> MASMTGGQQMGRDEAGITGTWYNQLGSTFIVTAGADGALTGTYESAVGNAESRYVLTGRYDSAPATDGSGTALGWTVAWKNNYRNAHSATTWSGQYVGGAQARINTQWLLTYGTTEANAWASTLVGHDTFTKVKPSAASIDAAKKAGVNNGNPLDAVQQ

Our work utilizes biotin–streptavidin (Sav) technology to develop artificial metalloproteins (ArMs) that mimic the active sites of natural copper metalloenzymes. Our group develops artificial metalloproteins (ArMs) using biotin–streptavidin (Sav) technology to mimic natural metalloenzyme active sites to characterize otherwise elusive intermediates and study the effects of the secondary coordination sphere on metal ion(s) reactivity. This approach leverages the strong binding affinity between biotinylated metal complexes and the Sav host to confine synthetic metal cofactors within a protein scaffold. By engineering ArMs with aromatic residues within their secondary coordination spheres, we systematically investigate the influence of these residues on Cu reactivity and oxidant activation. Our results demonstrate how the inclusion of aromatic residues within the secondary coordination sphere influences the structure and reactivity of copper ArMs.

We reasoned that a tyrosine mutation at position S112 would be close enough to our Cu cofactors to influence the structure and reactivity but would not be oriented to participate in direct coordination. To prepare this type of Cu ArM, a triple mutant variant of Sav, referred to as 2XM-S112Y-Sav, was engineered; this mutant contains S112Y and two additional mutations, K121A and E101Q, which we have found to prevent unwanted interactions with our artificial metallocofactors (S3 and Table S1†).21 We also utilized CuII-biot-et-dpa as our cofactor to assemble our ArMs, where (biot-et-dpa) is bis(2-pyridylmethyl)amine. One of the remaining coordination sites is occupied by an O atom donor from an acetate ion originating from our crystallization conditions and bound in a κ1-manner – this ligand is also H-bonded to a water molecule within the secondary coordination sphere. The final coordination site is occupied by an O/N donor from the N49 sidechain, which undergoes a conformational change to produce a previously unobserved rotamer (Fig. 2 and S4B†). Although protein crystallography cannot unambiguously discern the identity of the coordinating atom of the N49 sidechain (i.e., either O or N), we modelled the bound state as O-bound based on the pH of our crystallization conditions (pH = 6), which was below the pKa of the amide.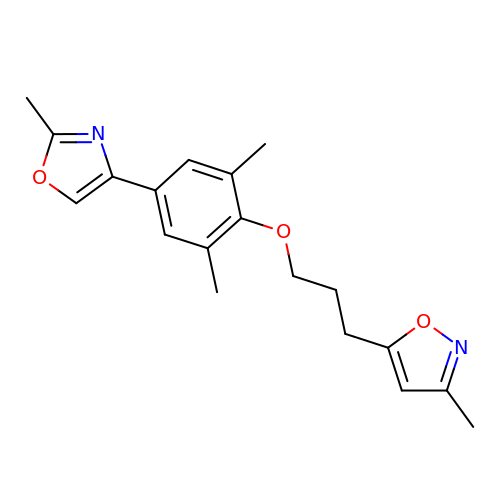2,6-DIMETHYL-1-(3-[3-METHYL-5-ISOXAZOLYL]-PROPANYL)-4-[2-METHYL-4-ISOXAZOLYL]-PHENOL | C19 H22 N2 O3 | SLPKYEWAKMNCPT-UHFFFAOYSA-N> MEVKKDNLSSQAKLWNFIYGFAESLVLKCAVQLDLANIIHNNGTSMTLSELSSRLPSQPVNEDALYRVMRYLVHMKLFTKASIDGELRYGLAPPAKFLVKGWDKCMVGSILAITDKDFMAPWHYLKDGLAGESGTAFEKALGMNIWGYMAEHP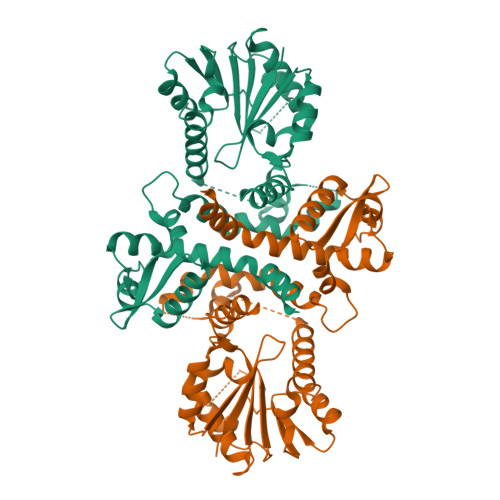EKNQLFNEAMANDSRLIMSALVKECGNIFNGITTLVDVGGGTGTAVRNIANAFPHIKCTVYDLPHVIADSPGYSEVHCVAGDMFKFIPKADAIMMKCILHDWDDKECIEILKRCKEAVPIEGGKVIIVDIVLNVQSEHPYTKMRLTLDLDMMLNTGGKERTEEEWKNLIHDAGYKGHKITQITAVQSVIEAYPY> MSIEIRKLSIEDLETLIEVARESWKWTYAGIYSEEYIESWIREKYSKE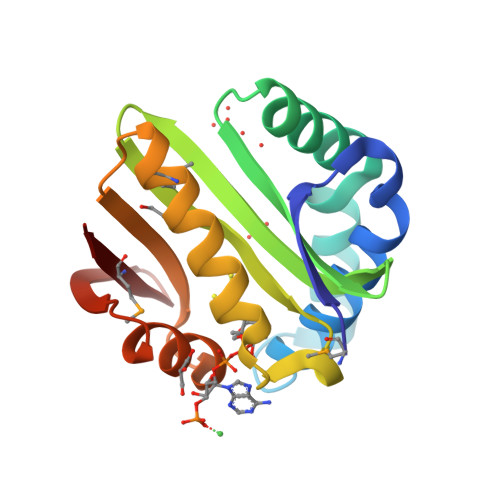KLLNEIVRSQSNLDILFLGAFADSTLIGFIELKIIANKAELLRLYLKPEYTHKKIGKTLLLEAEKIMKKKGILECRLYVHRQNSVGFSFYYKNGFKVEDTDGSDFIMEKKY> IVGGYECKPYSQPHQVSLNSGYHFCGGSLVNENWVVSAAHCYKSRVEVRLGEHNIKVTEGSEQFISSSRVIRH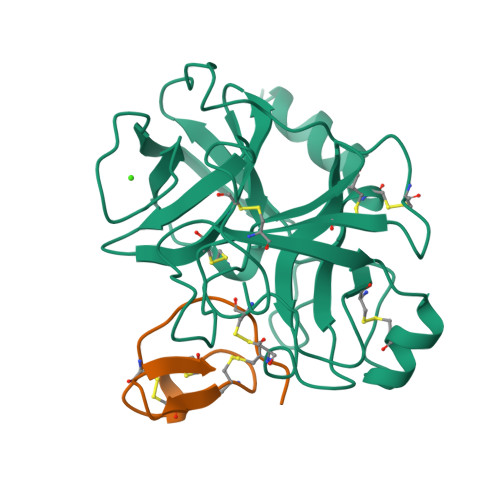PNYSSYNIDNDIMLIKLSKPATLNTYVQPVALPTSCAPAGTMCTVSGWGNTMSSTADSNKLQCLNIPILSYSDCNNSYPGMITNAMFCAGYLEGGKDSCQGDSGGPVVCNGELQGVVSWGYGCAEPGNPGVYAKVCIFNDWLTSTMASY;> RVCPKILMECKKDSDCLAECICLEHGYCG(2~{R},3~{R},4~{S},5~{R})-2-(6-aminopurin-9-yl)-5-[[4-[6-azanyl-9-[(2~{R},3~{R},4~{S},5~{R})-5-(hydroxymethyl)-3,4-bis(oxidanyl)oxolan-2-yl]purin-8-yl]but-3-ynylamino]methyl]oxolane-3,4-diol | C24 H29 N11 O7 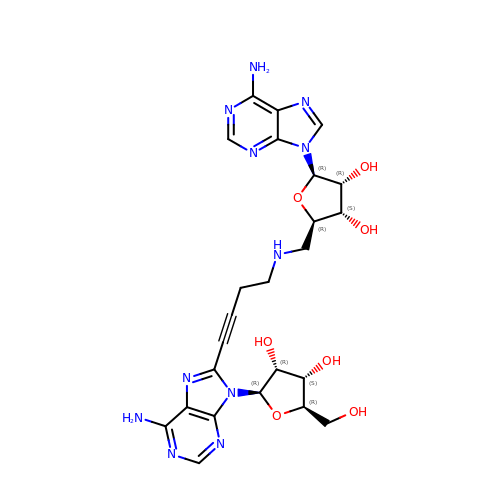| HUYGUSYCJOKUJB-KRSQEUQLSA-N>[4x]GPSDQVSLGVVGIGKIARDQHLPAIDAEPGFKLTACASRHAEVTGVRNYRDLRALLAAERELDAVSLCAPPQVRYAQARAALEAGKHVMLEKPPGATLGEVAVLEALARERGLTLFATWHSRCASAVEPAREWLATRAIRAVQVRWKEDVRRWHPGQQWIWEPGGLGVFDPGINALSIVTRILPRELVLREATLIVPSDVQTPIAAELDCADTDGVPVRAEFDWRHGPVEQWEIAVD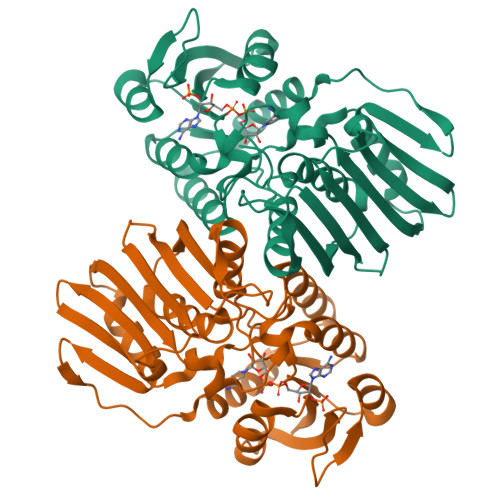TADGVLAISRGGAQLSIAGEPVELGPEREYPALYAHFHALIARGESDVDVRPLRLVADAFLFGRRVQTDAFGR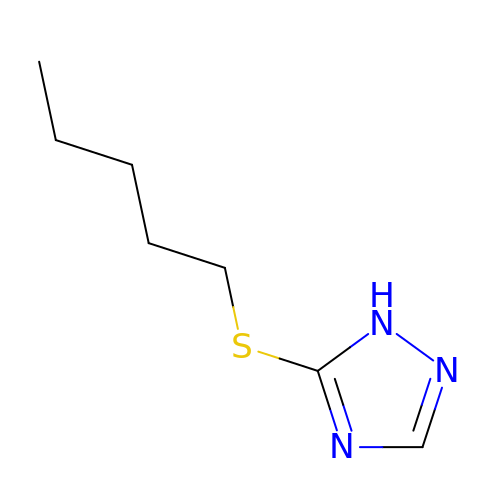5-(pentylsulfanyl)-1H-1,2,4-triazole | C7 H13 N3 S | YDSWCAZMHZEBFW-UHFFFAOYSA-N> MSPILGFWKIKGLVQPTRLLLEYLEEKYEEHLYERDEGDKWRNKKFELGLEFPNLPYYIDGDVKLTQSMAIIRYIADKHNMLGGCPKERAEISMLEGAVLDIRYGVSRIAYSKDFETLKVDFLSKLPEMLKMFEDRLCHKTYLNGDHVTHPDFMLYDALDVVLYMDPMCLDAFPKLVCFKKRIEAIPQIDKYLKSSKYIAWPLQGWQATFGGGDHP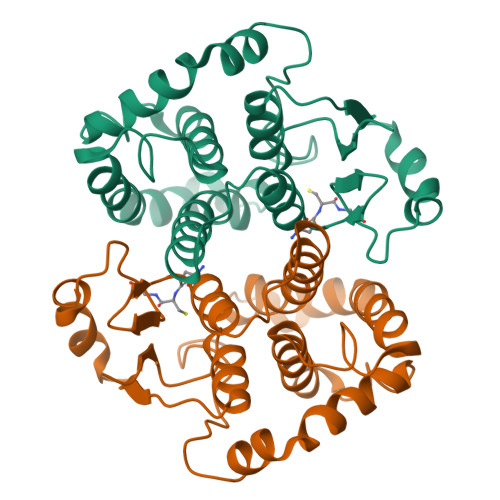PK> GMGSMSTPAASANGGQVLLLPFPAAQGHTNPMLQFGRRLAYHGLRPTLVTTRYVLSTTPPPGDPFRVAAISDGFDDASGMAALPDPGEYLRTLEAHGARTLAELLLSEARAGRPARVLVYDPAAPWARRVARAAGVATAAFLSQPCAVDLIYGEVCARRLALPVTPTDARGLYARGVLGVELGPDDVPPFVAAPELTPAFCEQSIEQFAGLEDDDDVLVNSFSDLEPKEAAYMESTWRAKTIGPSLPSFYLDDGRLRSNTAYGFNLFRSTVPCMEWLDKQPPRSVVLVSYGTVSTFDVAKLEELGNGLCNSGKPFLWVVRSNEEHKLSVQLRKKCEKRGLIVPFCPQLEVLAHKATGCFLSHCGWNSTLEAIVNGVPLVAMPHWADQPTISKYVESLWGMGVRVQLDKSGILQR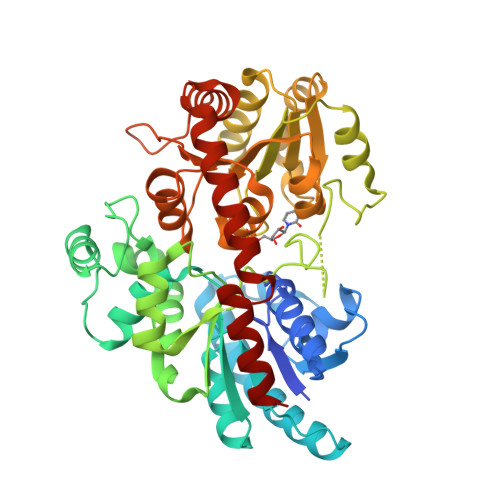EEVERCIREVMDGDRKEDYRRNATRLMKKAKESMQEGGSSDKNIAEFAAKYSN> GIPAPADNTVNIKTFDKVKNAFGDGLSQSAEGTFTFPADVTAVKTIKMFIKNECPNKTCDEWDRYANVYVKNKTTGEWYEIGRFITPYWVGTEKLPRGLEIDVTDFKSLLSGNTELKIYTETWLAKGREYSVDFDIVYGTPDYKYSAVVPVVQYNKSSIDGVPYGKAHTLALKKNIQLPTNT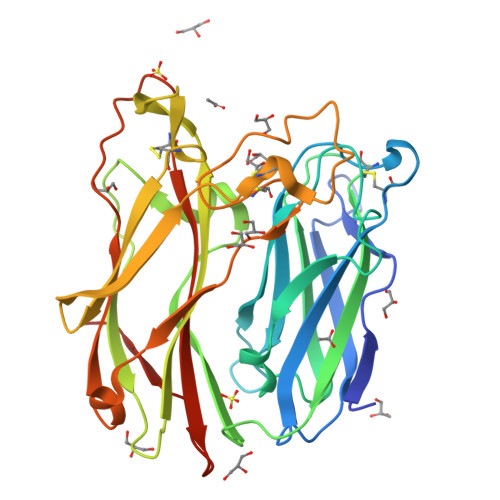EKAYLRTTISGWGHAKPYDAGSRGCAEWCFRTHTIAINNSNTFQHQLGALGCSANPINNQSPGNWTPDRAGWCPGMAVPTRIDVLNNSLIGSTFSYEYKFQNWTNNGTNGDAFYAISSFVIAKSNTPISAPVVTNLDPHHHHHH> MFFSRLSLSALKAAPAREALPGLLSRQSFSSAGFSQFSSQKFFFSPSRNFSQSPLF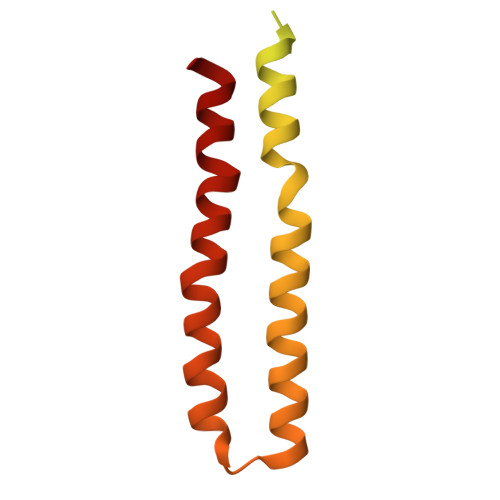QKHTPVHCNQRIASALVPTQQPAMTRQNPYAMQVGARYDAGVASLSAAIALMSVGGVAQGIGSLFAALVSGTARNPSIKEDLFTYTLIGMGFLEFLGIICVLMSAVLLYS5-methoxy-1,3-benzoxazole-2-carboxylic acid | C9 H7 N O4 | 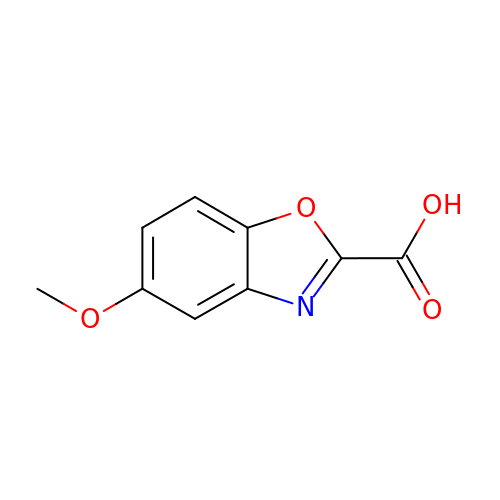SNQUKJWKYRHONV-UHFFFAOYSA-N> GEFTQSVSRLQSIVAGLKNAPSDQLINIFESCVRNPVENIMKILKGIGETFCQHYTQSTDEQPGSHIDFAVNRLKLAEILYYKILETVMVQETRRLHGMDMSVLLEQDIFHRSLMACCLEIVLFAYSSPRTFPWIIEVLNLQPFYFYKVIEVVIRSEEGLSRDMVKHLNSIEEQILESLAWSHDSALWEALQVSANKVPTCEEVIFPNNFETGNNRPKRTGSLALFYRKVYHLASVRLRDLCLKLDVSNELRRKIWTCFEFTLVHCPDLMKDRHLDQLLLCAFYIMAKVTKEERTFQEIMKSYRNQPQANSHVYRSVLLKSIKEERGDL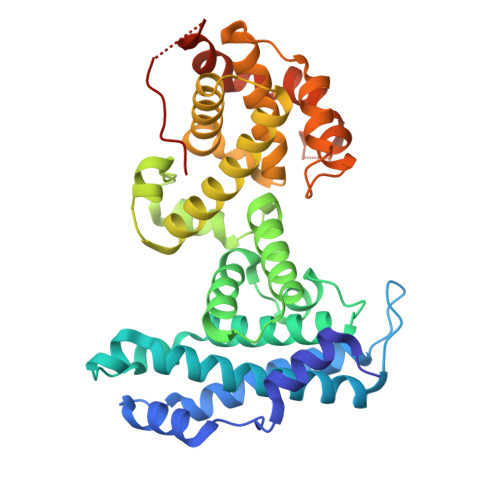IKFYNTIYVGRVKSFALKYDLANQDHMMDAPPLSPFPHIKQQ> MSTCPIDPPALRAAFAGPLDPQHAEVLLSRYDQHASRLLDALHALYGQRADYASWLAQWLGEVGDIARQRPQALQTLDSTRHAGWFGQPHMLGYSAYADRFAGTLQGVAERVPYLQELGVRYLHLLPFLRARAGDNDGGFAVSDYGQVEPSLGSNDDLVALTSRLREAGISLCADFVLNHTADDHAWAQAARAGDARYLDYYHHFADRTVPDRYEATLGQVFPHTAPGNFTWVDDTAQWMWTTFYPYQWDLNWSNPAVFGDMALAMLRLANLGVEAFRLDSTAYLW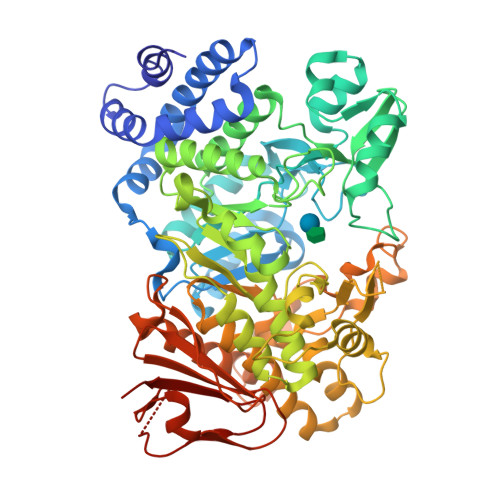KRIGTDCMNQSEAHTLLVALRAVTDIVAPAVVMKAQAIVPMTQLPPYFGSGVDEGHECHLAYHSTLMAAGWSALALQRGDILHNVIAHSPPLPRHCAWLSYVRCHDDIGWNVLQHEACGNAAQPPFSLRDVARFYANAVPGSYARGESFQSSGDGVHGTNGMAAALAGIQAAQEAGDAAALAVAVDRLVLLYAIALAMPGVPLIYMGDELAMVNDPGYRDDPHRQHEGRWLHRPAMDWQLAAQRHDAKSLSGTVYRRLRGLIRQRAALGALAADQALASIALNDPRVFALTRGDSFIALHNFSDQLLDVELAAIGVDGWTLLAIDDAIGGAAARGDGSIVLPPYGVRWLQRGTEHAPE>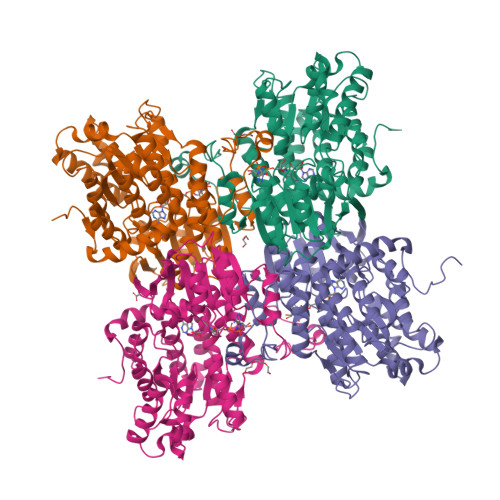[4x]GIDPFTMNAKPGFTDYIVKDIALADFGRKEISLAETEMPGLMATREEYGPKQPLKGARIAGSLHMTIQTAVLIETLAALGADIRWVSCNIYSTQDHAAAAIAAAGIPVFAVKGETLTEYWDYTAKLFDWHGGGTPNMILDDGGDATMLVHAGYRAEQGDTAFLDKPGSEEEEIFYALVKRLLKEKPKGWFAEIAKNIKGVSEETTTGVHRLYEMANKGTLLFPAINVNDSVTKSKFDNLYGCRESLVDGIRRGTDVMLSGKVAMVAGFGDVGKGSAASLRQAGCRVMVSEVDPICALQAAMEGYEVVTMEDAAPRADIFVTATGNKDIITIEHMRAMKDRAIVCNIGHFDNEIQIASLRNLKWTNIKPQVDEIEFPDKHRIIMLSEGRLVNLGNAMGHPSFVMSASFTNQTLAQIELFANNKDSKYAKKVYVLPKTLDEKVARLHLAKIGVKLTELRKDQADYIGVKQEGPYKSDHYRY>MKSPIPLRDVPQSNIFRKGDVFVLFGELFGRGYANGLINEARDAGMTIVGITVGRRDENNALRALTAEELATAEANLGGRIINVPLMAGFDLDAPAGEPTPTDLLADMTLKSWQDDKLDWAHIEKCRAVGVQRFKDGVAKVMAELDGMIPDGANAFFAHTMAGGIPKVKVFLAIANRIYKGRGERFLSSSALLNSDLGKLILMNFDEVTANTFLHLIEGSAAIRARLEKSGGQVRYSAYGYHGTEILIDDKYQWQTYTSYTQGKAKMRLERIAEDAWKQGIKATVY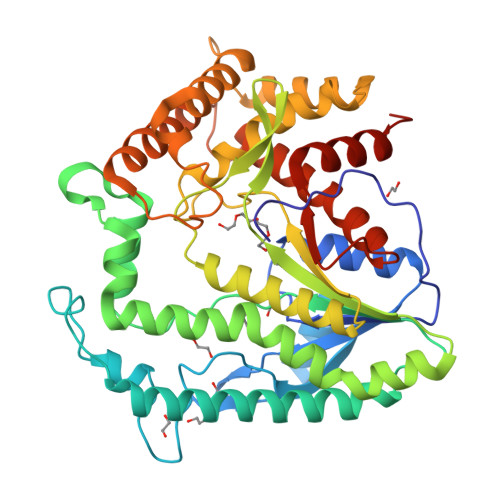NCPEIRTNSSDIFVGVELSLFPLLKALKKENGGAWAEAQWQACREVLSEGHTLESLLQKIDDYNASDVMKGFRNFEAWPMPNTAELADIMIGTSDEITKMHKSRDALVTDVLSALVLEGTGPLMFHESSNPAGPVLWLSHDVIAKQLNLMHRLEHHHHHH[3x]> TQKSLSKEEIERYSRQMIVPGMGKEGQLRLMNAKVLIIGAGGLGCPAAQYLAGAGVGTIGIVDGDSVETSNLHRQVAHATKRVGMLKVDSLITHLIEINPLPVYVPYRFDLTPQNAAQIIKPWDVILDCTDNPATRYLISDVCVLLGKPLVSAASVQKSGQLIVLNCPPTPQGVVNKKAAPCYRCCFKKPPPPSAQTSKGE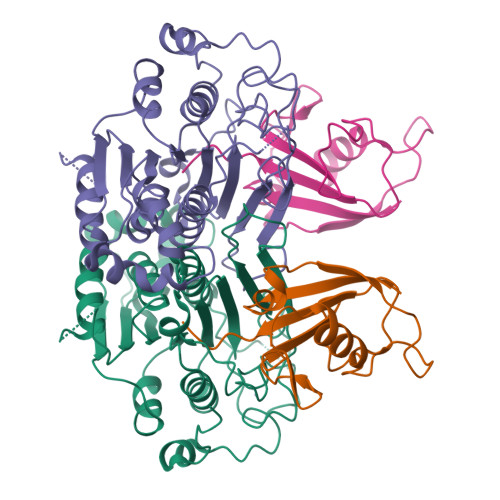AGIMGPVVGMMGVAQAGEAIKILVSQLHMPPKEGEEVSPEKNLVQPTLLIYTYDLNSAIGPYSFRALKMGGRKKDCFACGENSTLTLDGIKSGNPNYVQQ;> IPITVDFSGGLEMLFDNQRRHSISLPAKDTEGKPVTIAFLIDYICKKLMKDPRTDLFVLDNHIRPGILVLINDADWELEGEEAYEIQPNDNILFVSTLHGG>[4x]MKHHHHHHPMGPRDVALGSSIISIKNQALGGA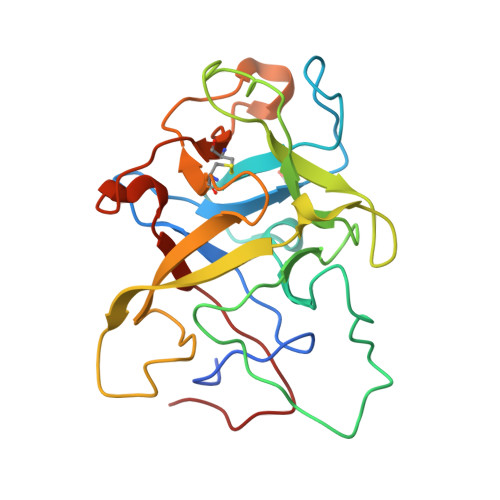LLHSHVQPFPEGSEQQQVTVYGYSDANNEWFFQRIRGVEPWTDAENKTIEFVKGGEMYRLMHRLTGKNLHTHEVPAPISKSEYEVSAYGDVDLGDYKDNWIIEIVEQVGEEDPTLLHPLSTSFRIKNSILGCYLAQSGKHLPEWGFRQGEVVCLKHASKRDKRTWWNIETHENERLPQGE>[2x]MSREEVESLIQEVLEVYPEKARKDRNKHLAVNDPAVTQSKKCIISNKKSQPGLMTIRGCAYAGSKGVVWGPIKDMIHISHGPVGCGQYSRAGRRNYYIGTTGVNAFVTMNFTSDFQEKDIVFGGDKKLAKLIDEVETLFPLNKGISVQSECPIGLIGDDIESVSKVKGAELSKTIVPVRCEGFRGVSQSLGHHIANDAVRDWVLGKRDEDTTFASTPYDVAIIGDYNIGGDAWSSRILLEEMGLRCVAQWSGDGSISEIELTPKVKLNLVHCYRSMNYISRHMEEKYGIPWMEYNFFGPTKTIESLRAIAAKFDESIQKKCEEVIAKYKPEWEAVVAKYRPRLEGKRVMLYIGGLRPRHVIGAYEDLGMEVVGTGYEFAHNDDYDRTMKEMGDSTLLYDDVTGYEFEEFVKRIKPDLIGSGIKEKFIFQKMGIPFREMHSWDYSGPYHGFDGFAIFARDMDMTLNNPCWKKLQAPWE;>[2x]SQQVDKIKASYPLFLDQDYKDMLAKKRDGFEEKYPQDKIDEVFQWTTTKEYQELNFQREALTVNPAKACQPLGAVLCALGFEKTMPYVHGSQGCVAYFRSYFNRHFREPVSCVSDSMTEDAAVFGGQQNMKDGLQNCKATYKPDMIAVSTTCMAEVIGDDLNAFINNSKKEGFIPDEFPVPFAHTPSFVGSHVTGWDNMFEGIARYFTLKSMDDKVVGSNKKINIVPGFETYLGNFRVIKRMLSEMGVGYSLLSDPEEVLDTPADGQFRMYAGGTTQEEMKDAPNALNTVLLQPWHLEKTKKFVEGTWKHEVPKLNIPMGLDWTDEFLMKVSEISGQPIPASLTKERGRLVDMMTDSHTWLHGKRFALWGDPDFVMGLVKFLLELGCEPVHILCHNGNKRWKKAVDAILAASPYGKNATVYIGKDLWHLRSLVFTDKPDFMIGNSYGKFIQRDTLHKGKEFEVPLIRIGFPIFDRHHLHRSTTLGYEGAMQILTTLVNSILERLDEETRGMQATDYNHDLVR

Nitrogenase catalyzes the ATP-dependent reduction of dinitrogen to ammonia during the process of biological nitrogen fixation that is essential for sustaining life. The Fe-protein mediates ATP-dependent electron transfer (ET) through its [4Fe:4S] cluster to the intermediate [8Fe:7S] P-cluster in the MoFe-protein; the electrons are subsequently shuttled to a [7Fe:1Mo:9S:1C]-R-homocitrate metallocluster, the FeMo-cofactor, within the active site of the MoFe-protein. The active site FeMo-cofactor contains a [7Fe:1Mo:9S:1C] metallocluster coordinated with an R-homocitrate (HCA) molecule.

A resulting 2.37 Å resolution structure of MoFeAlkaline-inactivated demonstrates that HCA is lost from the active site under these conditions. In contrast, the MoFeAlkaline-inactivated cryoEM structure exhibited asymmetric disorder within one α-subunit, which likely stems from the averaging of heterogeneous intermediate states. This poor density corresponds to residues 1–48, 354–360, 376–416, and 423–425, which lack traceable density in the more disjointed α-subunit (2.37 Å resolution). In the MoFeAlkaline-inactivated structure, both P-cluster ligands and one FeMo-cofactor appear well ordered, but within the active site of the disordered α-subunit, the density corresponding to the crystallographic location of FeMo-cofactor appears distorted. The disordered active site clearly lacks density for HCA, while the ordered active site shows reduced density at the HCA coordination site. Within both αβ dimers of the MoFeAlkaline-inactivated state, Phe α300 experiences a rotamer rearrangement with respect to the MoFeAs-isolated and MoFeAlkaline states. The movement of this bulky side chain within the disordered dimer is coupled with altered positioning of three histidines, His α274, His α362, and His α451, towards a coordination site for an unidentified ligand ~8 Å from the terminal Fe1 of the FeMo-cofactor. In addition, while density around the FeMo-cofactor is poorly resolved, a rearrangement of the His α442 loop that normally ligates the FeMo-cofactor can be partially traced into smoothed maps and may also participate in this coordination in a tetrahedral fashion. Given the nature of the density and the geometry of the coordination, the bound ligand could be metal. Interestingly, the Trp α253 flip is observed in both α-subunits in MoFeAlkaline-inactivated, where previously it was observed only in one subunit under turnover conditions.>[2x]GMTKLPATSDIYISFFMFTTNLQPDNLDYRRIVVAHIKKLQRFGYSGFEFPIAPGLPE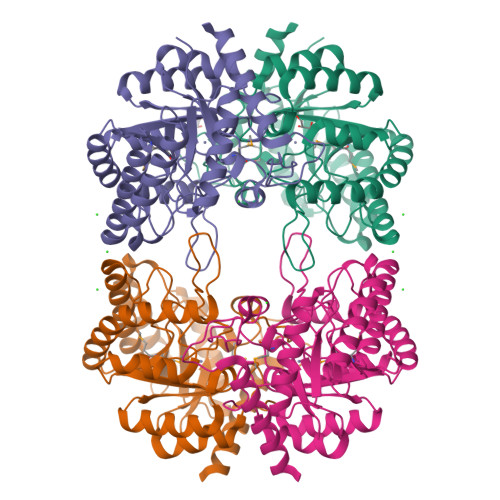NYAQDLENYTNLRHYLDSEGLENVKISTNVGATRTFDPSSNYPEQRQEALEYLKSRVDITAALGGEIMMGPIVIPYGVFPTTDFNEPIWSDELQEHLKVRYANAQPILDKLGEYAEIKKVKLAIEPITHWETPGPNKLSQLIEFLKGVKSKQVGVVIDSAHEILDGEGPEIFKTQVEYLAQQGRLHYVQVSPPDRGALHTSWLPWKSFLTPIVKVYDGPIAVEIFNAIPAFTNSLRLTRRKFWIPDEDPPNQYPNAYDIADEAIKVTRKELKKIGSK> AYTTAQLVTAYTNANLGKAPDAATTLTLDAYATQTQTGGLSDAAALTNTLKLVNSTTAVAIQ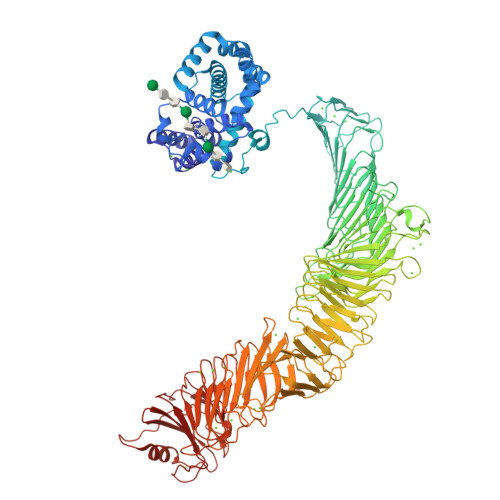TYQFFTGVAPSAAGLDFLVDSTTNTNDLNDAYYSKFAQENRFINFSINLATGAGAGATAFAAAYTGVSYAQTVATAYDKIIGNAVATAAGVDVAAAVAFLSRQANIDYLTAFVRANTPFTAAADIDLAVKAALIGTILNAATVSGIGGYATATAAMINDLSDGALSTDNAAGVNLFTAYPSSGVSGSTLSLTTGTDTLTGTANNDTFVAGEVAGAATLTVGDTLSGGAGTDVLNWVQAAAVTALPTGVTISGIETMNVTSGAAITLNTSSGVTGLTALNTNTSGAAQTVTAGAGQNLTATTAAQAANNVAVDGGANVTVASTGVTSGTTTVGANSAASGTVSVSVANSSTTTTGAIAVTGGTAVTVAQTAGNAVNTTLTQADVTVTGNSSTTAVTVTQTAAATAGATVAGRVNGAVTITDSAAASATTAGKIATVTLGSFGAATIDSSALTTVNLSGTGTSLGIGRGALTATPTANTLTLNVNGLTTTGAITDSEAAADDGFTTINIAGSTASSTIASLVAADATTLNISGDARVTITSHTAAALTGITVTNSVGATLGAELATGLVFTGGAGADSILLGATTKAIVMGAGDDTVTVSSATLGAGGSVNGGDGTDVLVANVNGSSFSADPAFGGFETLRVAGAAAQGSHNANGFTALQLGATAGATTFTNVAVNVGLTVLAAPTGTTTVTLANATGTSDVFNLTLSSSAALAAGTVALAGVETVNIAATDTNTTAHVDTLTLQATSAKSIVVTGNAGLNLTNTGNTAVTSFDASAVTGTGSAVTFVSANTTVGEVVTIRGGAGADSLTGSATANDTIIGGAGADTLVYTGGTDTFTGGTGADIFDINAIGTSTAFVTITDAAVGDKLDLVGISTNGAIADGAFGAAVTLGAAATLAQYLDAAAAGDGSGTSVAKWFQFGGDTYVVVDSSAGATFVSGADAVIKLTGLVTLTTSAFATEVLTLA> ALVKEEIQAKEYLENLNKELAKRTNVETEAAWAYGSNITDENEKKKNEISAELAKFMKEVASDTTKFQWRSYQSEDLKRQFKALTKLGYAALPEDDYAELLDTLSAMESNFAKVKVCDYKDSTKCDLALDPEIEEVISKSRDHEELAYYWREFYDKAGTAVRSQFERYVELNTKAAKLNNFTSGAEAWLDEYEDDTFEQQLEDIFADIRPLYQQIHGYVRFRLRKHYGDAVVSETGPIPMHLLGNMWAQQWSEIADIVSPFPEKPLVDVSAEMEKQGYTPLKMFQMGDDFFTSMNLTKLPQDFWDKSIIEKPTDGRDLVCHASAWDFYLTDDVRIKQCTRVTQDQLFTVHHELGHIQYFLQYQHQPFVYRTGANPGFHEAVGDVLSLSVSTPKHLEKIGLLKDYVRDDEARINQLFLTALDKIVFLPFAFTMDKYRWSLFRGEVDKANWNCAFWKLRDEYSGIEPPVVRSEKDFDAPAKYHISADVEYLRYLVSFIIQFQFYKSACIKAGQYDPDNVELPLDNCDIYGSAAAGAAFHNMLSMGASKPWPDALEAFNGERIMSGKAIAEYFEPLRVWLEAENIKNNVHIGWTTSNKCVS;> DRVYIHPF

Peptidyl dipeptidase A is a highly glycosylated ectoenzyme that cleaves dipeptides from the C-terminus of a broad range of oligopeptides. AnCE is a single-domain glycosylated protein that closely shares enzymatic properties with human ACE (in particular the C-domain of human somatic ACE) and is inhibited by classic inhibitors of the human enzymes 14–17. In this study, we elucidate how the natural peptides Ang II (the principal end-product of the renin-angiotensin–aldosterone system), Arg–Pro–Pro (the BK-derived peptide) and bradykinin-potentiating peptide-b (BPPb, a snake venom inhibitor) bind to the active site of AnCE, revealing novel interactions involving several enzyme subsites. Comparison of the four structures clearly shows a common mode of peptide binding to AnCE.

The co-crystallization of Ang I (Asp–Arg–Val–Tyr–Ile–His–Pro–Phe–His–Leu) with AnCE resulted in conversion to Ang II (Asp–Arg–Val–Tyr–Ile–His–Pro–Phe) which can be observed in the substrate-binding channel. In the AnCE–Ang II peptide complex structure, clear electron density was observed for the tetrapeptide Tyr–Ile–His–Pro. In the case of AnCE–Ang II peptide complex, the observable part of the Ang II peptide docked with residues P2, P1, P1′ and P2′, occupying the S2, S1, S1′ and S2′ subsites, respectively. In this configuration, the peptide could not be cleaved, suggesting that Ang II is a true competitive inhibitor of AnCE-mediated conversion of Ang I. The C-terminal Pro residue (P2′) is clearly visible and anchors the peptide at the S2′ subsite by hydrogen bonds with three residues (Gln265, Tyr504 and Lys495), whereas the pyrrolidine ring is stabilized through hydrophobic interaction with the surrounding aromatic residues (in particular Tyr507 and Phe441). The main chain of the His (P1′) residue from the Ang II peptide makes hydrogen bond interactions with His337 and His497. At the P1 position, the Ile residue is involved in a tetrahedral coordination with the zinc ion and stabilized by a hydrogen bond with Tyr507. The visible electron density terminates at the P2 position with the main chain of Tyr strongly interacting with the main chain of Ala340 (through two hydrogen bonds). The hydroxyl group of Tyr interacts with Thr387 of AnCE. Ang II is resistant to hydrolysis by AnCE and repositions itself in the active site so that the penultimate C-terminal Pro residue shifts from S2 to the S2′ subsite after the hydrolysis of Ang I. Based on molecular modelling, we predict that the C-terminal Phe of Ang II could be accommodated in the binding pocket. The crystal structure of AnCE in complex with Ang II provided direct structural evidence for Ang II being a competitive inhibitor of AnCE activity.> MVAKFQPPPEYQLTAAELKQIVDQSLSGGDLACRLLVQLFPELFSDVDFS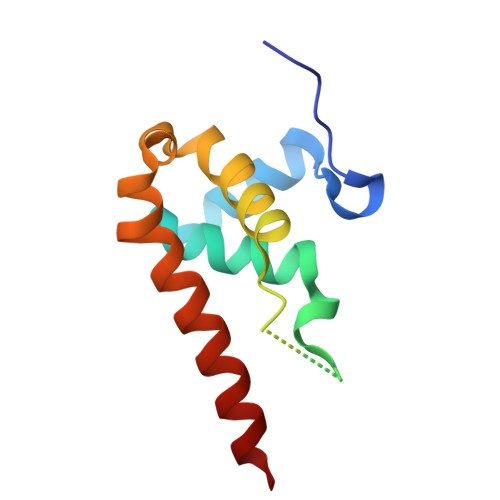RGCSACGFAAKRKLESLHLQLIRNYVEVYYPSVKDTAVWQAECLPQLNDFFSRFWAQREMED>[14x]MIANE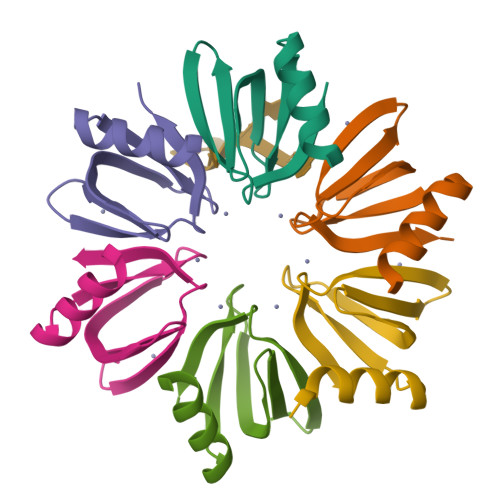NIQDKALENFKANQTEVTVFFLNGFQMKGVIEEYDKYVVSLNSQGKQHLIYKHAISTYTVETEGQASTESEE>YHEEFARAGKQAGLQVWRIEKLELVPVPQSAHGDFYVGDAYLVLHTAKTSRGFTYRLHFWLGKECSQDESTAAAIFTVQMDDYLGGKPVQNRELQGYESNDFVSYFKGGLKYKAGGVASGLNHVLTNDLTAKRLLHVKGRRVVRATEVPLSWDSFNKGDCFIIDLGTEIYQWCGSSCNKYERLKANQVATGIRYNERKGRSELIVVEEGSEPSELIKVLGEKPELPDGGDDDDIIADISNRKMAKLYM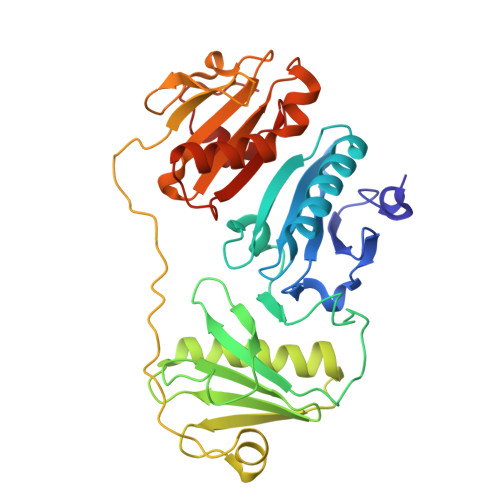VSDASGSMRVTVVAEENPFSMAMLLSEECFILDHGAAKQIFVWKGKDANPQERKAAMKTAEEFLQQMNYSKNTQIQVLPEGGETPIFKQFFKDWRD[2x]> GHMASATARVRIYPLALAKVVKHAASSLQREVAGLLVGKSAGKVLEIWDAVTGEQYGTPAYVQLDEMVMAKVAEELSKSDKNLYIVGWYHSHPGLDVFLSPTDIDTQKRYQAMFSKAVALVVDPVDYAKTRRISSLKFKVFQISKEGRVVSLPVS

The first complete archaeal Ub modifier system, including E2 and E3 enzymes, was discovered in 2011 in Candidatus Caldiarchaeum subterraneum. C. subterraneum Ub (CsUb), E1, E2, and E3 are organized in a single operon, adjacent to a second E3 protein and a JAMM protease (CsRpn11) with high sequence similarity to eukaryotic Rpn119. We have shown that CsRpn11 is highly active on its own, cleaving both CsUb precursors and, at a later stage of the ubiquitination cascade, CsUb-conjugated substrate proteins. Our bioinformatic, structural, and biochemical results reveal unique features of the archaeal proteins, but also remarkable conceptual similarities with their eukaryotic counterparts.

To determine crystal structures for CsRpn11, we used the full-length wild-type form and a series of truncated proteins with deletions C-terminal of the JAMM core domain. Using these constructs, we obtained crystals for full-length CsRpn11 and truncated CsRpn11Δ149–202, for which we collected data to 1.65 Å and 1.35 Å resolution. We located two protomers in the asymmetric unit, which form a homodimer grossly reminiscent of the Rpn8–Rpn11 heterodimer. However, while the latter is assembled in an antiparallel fashion, the CsRpn11 homodimer is parallel, with an interface formed by the first and the fourth alpha-helix, H1 and H4, of CsRpn11. In the truncated CsRpn11Δ149–202 structure, however, which is lacking H4, and which we solved on the basis of the full-length Rpn11 coordinates, this dimerization is not observed. At 45 °C, truncated CsRpn11 processed CsUb-pre with a KM of 24.2 µM and a kcat of 3.5 min−1, and bound the reaction product with a KD of 14.6 µM. With a KM of 31.6 µM and a kcat of 4.0 min−1, the full-length version displayed similar reaction parameters, indicating that the CsRpn11 C-terminal helices are indeed not critically required for catalysis.>[3x]MGSDKIHHHHHHENLYFQG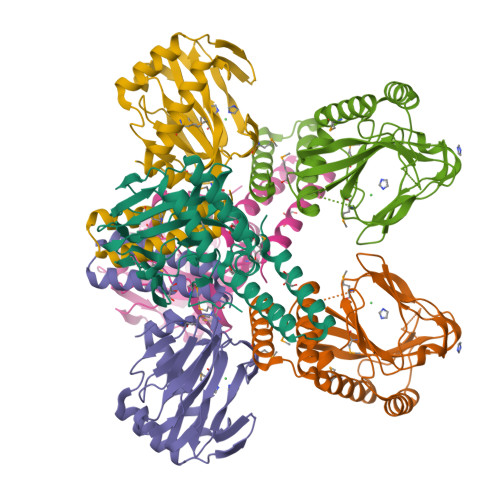MLIEIPNVFSKQEVSHLREQLDARRWIDGNQTSGAMATTRKRNQQLDKDDPVAVALGQQIMDRLLAHPQFVSAALPLQFYPPLFNRYQGGETFGYHIDNAIRSTPDGMIRTDLSATLFLSEPENYQGGELVIQDTYGQQSIKLSAGSLVLYPSSSLHQVTPVLSGERTAAFMWLQSMVRDEGQRRLLFQLDQSIQSLTAQTAAEQELFNLSGVYHNLLRRWSEL The acyl-ACP synthetase (termed AasS) of the zoonotic pathogen Vibrio harveyi recycles exogenous fatty acid (eFA), bypassing the requirement of type II fatty acid synthesis (FAS II), a druggable pathway. Very recently, the AasS (533 aa) of V. harveyi was found to feature a large domain at N-terminus (termed AasS_N) that is connected with a compact C-terminal domain by a flexible linker. As expected, a hexamer ring-like overall structure was invariantly formed in all the three types of AasS particles, regardless of a cofactor/inhibitor. Obviously, the pattern of AasS oligomerization is recognized as a trimer of dimers, which mainly relies on two interfaces constituted by the AasS_N domain.

We solved two high-resolution cryo-EM structures of AasS liganded with C10-AMS inhibitor (2.33 Å) and C10-AMP intermediate (2.19 Å) in addition to its apo form (2.53 Å). The decanoic acid (C10) as a favorable substrate, can be converted into C10-AMP by AasS enzyme. The occupancy of C10-AMP intermediate renders the AasS_C domain (colored hot-pink) in an ‘open’ orientation. As for the cavity for C10-AMP occupancy, a C10-AMP molecule contacts several AasS_C active site. In brief, an adenine base is held in place by the hydrophobic side chains of Y318 and I423, and the ribose hydroxyl groups form a hydrogen bond network with the two residues (D411 and R426). The K522 residue from the AasS_C domain interacts with the ribose ring oxygen atom and the bridging oxygen atom of AMP via two hydrogen bonds. The AMP phosphate is coordinated by a Mg2+ atom as well as the hydroxyl groups of S321. The carbonyl group of C10-AMP gives a hydrogen bond with H226 site. The hydrophobic carbon chain of C10 is fixed in place by the four residues (V293, I326, I329, and the conserved W230). Notably, the W230 residue plays a gatekeeper role in eFA loading by AasS, which is equivalent to the W234 of ttFACS.

>[6x]MNQYVNDPSNYQLLIKNLLFSPVAFNPEQEIVYANHRRHSYKTFHDRVRQFANALTKMGVKKGDTVAVMDYDSHRYLECYFAIPMIGAKLHMINVRLSPEQILYTIDHAEDDIILIHEEFLPILDQIKGRIDTVTRYVVLRDDEECEYERLLEQESTEYNFPDFDENTVATTFYTTGTTGFPKGVFFTHRQLVLHTMGILSTIGTNASQGRLHQGDIYMPITPMFHVHAWGLPYMATMLGVKQVYPGKYVPDVLLNLIEQEKVTFSHCVPTILHLLLSSPKSKAMDFSGWKVVIGGAALPKALCKSALERDIDVFAGYGMSETGPILSIVQLTPEQLELDVDQQAEYRSKTGKKVALVEAYIVDEDMNKLPHDGETAGEIVVRAPWLTPNYYKDNKNSKALWRGGYLHTGDVAHIDDEGFIKITDRVKDMIKISGEWVSSLELEDILHQHQSVSEVAVIGMPHNKWGEVPLALVTLKEDAQVTEKELLGFAKDFINKGILAREALLLKVKIVDEIAKTSVGKVDKKELRKLHL4,4'-DIACETYLDIPHENYLUREA-BIS(GUANYLHYDRAZONE) 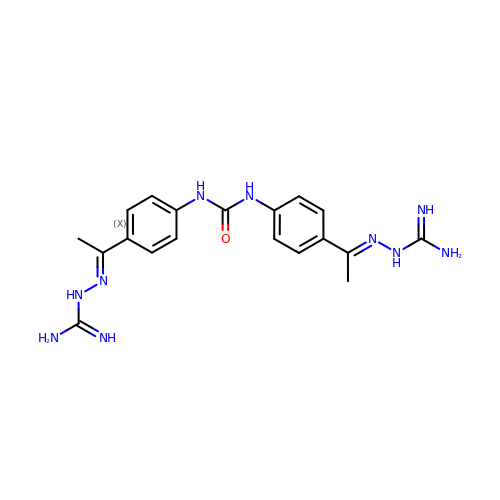| C19 H24 N10 O | HCAQGQIHBFVVIX-LYXAAFRTSA-N>SMFEIKKICCIGAGYVGGPTCSVIAHMCPEIRVTVVDVNESRINAWNSPTLPIYEPGLKEVVESCRGKNLFFSTNIDDAIKEADLVFISVNTPTKTYGMGKGRAADLKYIEACARRIVQNSNGYKIVTEKSAVPVRAAESIRRIFDANTKPNLNLQVLSNPEFLAEGTAIKDLKNPDRVLIGGDETPEGQRAVQALCAVYEHWVPREKILTTNTWSSELSKLAANAFLAQRISSINSISALCEATGADVEEVATAIGMDQRIGNKFLKASVGFGGSCFQKDV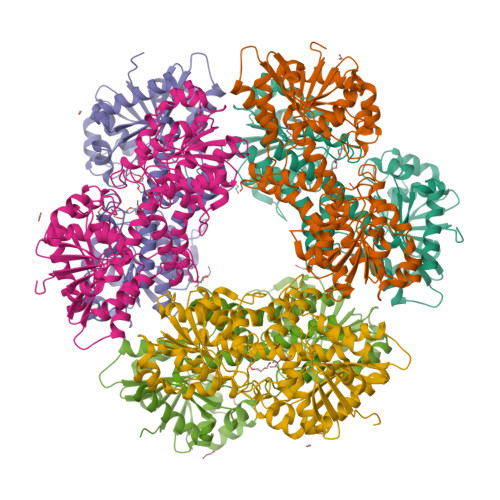LNLVYLCEALNLPEVARYWQQVIDMNDYQRRRFASRIIDSLFNTVTDKKIAILGFAFKKDTGDTRESSSIYISKYLMDEGAHLHIYDPKVPREQIVVDLSHPGVSEDDQVSRLVTISKDPYEACDGAHAVVICTEWDMFKELDYERIHKKMLKPAFIFDGRRVLDGLHNELQTIGFQIETIGKKV[6x]>MTISNLLKQRVRYAPYLKKVKEAHELIPLFKNGQYLGWSGFTGVGTPKAVPEALIDHVEKNNLQGKLRFNLFVGASAGPEENRWAEHDMIIKRAPHQVGKPIAKAINQGRIEFFDKHLSMFPQDLTYGFYTRERKDNKILDYTIIEATAIKEDGSIVPGPSVGGSPEFITVSDKVIIEVNTATPSFEGIHDIDMPVNPPFRKPYPYLKVDDKCGVDSIPVDPEKVVAIVESTMRDQVPPNTPSDDMSRAIAGHLVEFFRNEVKHGRLPENLLPLQSGIGNIANAVIEGLAGAQFKHLTVWTEVLQDSFLDLFENGSLDYATATSVRLTEKGFDRAFANWENFKHRLCLRSQVVSNNPEMIRRLGVIAMNTPVEVDIYAHANSTNVNGSRMLNGLGGSADFLRNAKLSIMHAPSARPTKVDPTGISTIVPMASHVDQTEHDLDILVTDQGLADLRGLSPKERAREIINKCAHPDYQALLTDYLDRAEHYAKKHNCLH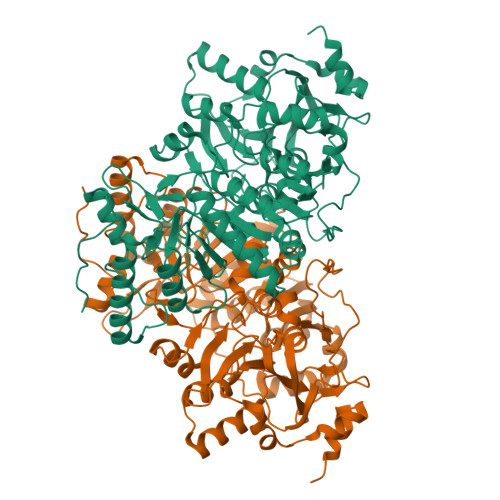EPHMLKNAFKFHTNLAEKGTMKVDSWEPVD[2x]> MHHHHHHENLYFQGAAYLSRIQRGGHIQPFGCTLAVADDSSFRLLAFSENAADLLDLSPHHSVPSLDSAAPPPVSLGADARLLFSPSSAVLLERAFAAREISLLNPLWIHSRVSSKPFYAILHRIDVGVVIDLEPARTEDPALSIAGAVQSQKLAVRAISRLQALPGGDIKLLCDTVVEHVRELTGYDRVMVYRFHEDEHGEVVAESRRDNLEPYLGLHYPATDIPQASRFLFRQNRVRMIADCHATPVRVIQDPGMSQPLCLVGSTLRAPHGCHAQYMANMG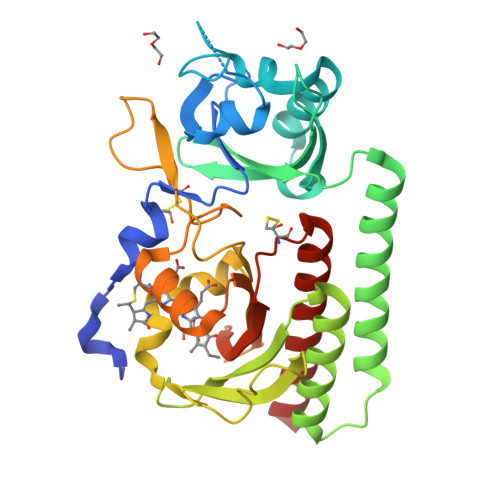SIASLVMAVIISSGGDDEQTGRGGISSAMKLWGLVVCHHTSPRCIPFPLRYACEFLMQAFGLQLNMELQL The HIV-1 Trans-Activation Response element (TAR) RNA, located at both ends of its RNA genome, is one of the most conserved RNA structural elements in retroviruses. It assumes multiple, dynamic conformations to carry out critical functions in several stages of the HIV-1 life cycle, including reverse transcription, proviral transcription, genome dimerization and packaging, viral translation, and immune suppression, etc. Here, we report crystal structures of the full-length HIV-1 TAR which reveal substantial conformational mobility in its three conserved bulges and in its lower stem, which coordinately maintain the structural fluidity of the entire RNA. We find that TAR RNA is a robust inhibitor of PKR, and primarily uses its lower stem to capture and sequester PKR monomers, preventing their dimerization and activation.

Interestingly, soaking the TAR-II crystals with CaCl2 stabilized the extrahelical UCU bulge, and promoted a U23-C24 stacking interaction. This is apparently mediated by Ca2+ coordination with the juxtaposed RNA backbone phosphate oxygens of the bulge. Similar effects of Ca2+ were also observed in a previous mini-TAR crystal structure. These findings suggest that the distinctive structural, electrostatic, and chemical environment of the UCU bulge, especially its distorted backbone, can create specific cation-binding sites. In turn, binding by divalent cations such as Mg2+ and Ca2+ can also modulate the conformation of this flexible RNA bulge. For comparison, Mg2+ and Ca2+ also remodel the bulge but are insufficient to drive stable triple formation.

> GGUCUCUCUGGUUAAGCCAGAUCUGAGCCGAAAAGCUCUCUGGCUAACUAGGGAACC> MIGMAEVKLINIWKRFGDVTAVKDLSLEIKDGEFLVLLGPSGCGKTTTLRMIAGLEEPTRGQIYIEDNLVADPEKGVFVPPKERDVAMVFQSY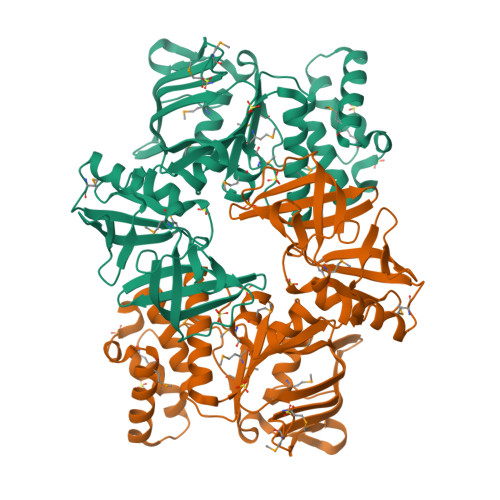ALYPHMTVYDNIAFPLKLRKVPKQEIDKRVREVAEMLGLTELLNRKPRELSGGQRQRVALGRAIIRRPKVFLMDEPLSNLDAKLRVKMRAELKKLQRQLGVTTIYVTHDQVEAMTMGDRIAVMNKGELQQVGTPDEVYYKPVNTFVAGFIGSPPMNFLDATITDDGFLDFGEFKLKLLQDQFEVLEEENMVGKEVIFGIRPEDVHDASFTHIDVPEENTVKATVDIIENLGGEKIVHLRRGNISFTAKFPKESKVREGDEVSVVFDMKKIHIFRKDTEKAIF> GLPTELRPGTNQFLTTEDDTAAPILPGFSPTPSIHIPGEVRSLLELCRVETILEVNNTTDATGLNRLLIPVSAQNKADELCAAFMVDPGRIGPWQSTLVGQICRYYTQWSGSLKVTFM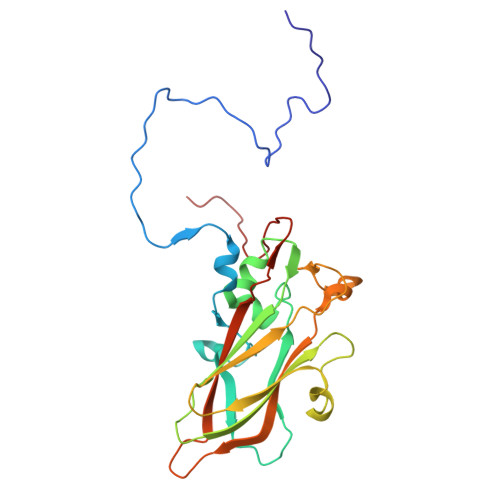FTGSFMATGKMLIAYSPPGSAQPANRETAMLGTHVIWDFGLQSSVSLVIPWISNTHFRTAKTGGNYDYYTAGVVTLWYQTNYVVPPETPGEAYIIAMGAAQDNFTLKICKDTDEVTQQAVLQ>SAPVELVAQPVNAQILPEGEPATPMLGFNGGTPGPVLRARQGEVFDIRFQNQIGEGSAVHWHGLRIDNAMDGVPGMTQDVVEAGGEFEYSFRAPDAGTFWYHSHNRSWEQVAKGLYGPLIVEEPTPPDVDHDLIIMIDDWRITENGVLADGFENMRDQAHQGRLGNFARALVEPVTPVRRGDRV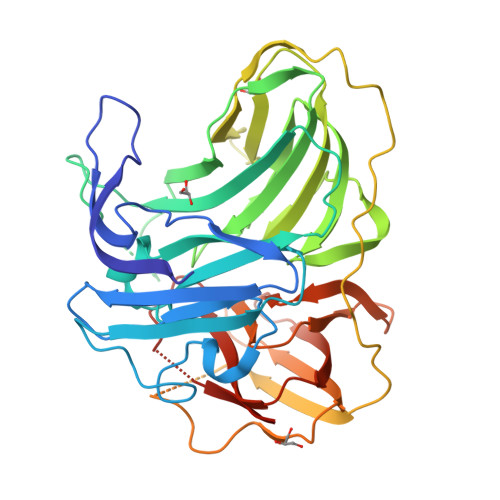RLRLINVATDRIFPVELEGVEGKVVALDGMPIVDPQEFSGLILAPAQRADIIADVITDAPIGFVFPTRDGPYLLGEIPVKGANTTRQPSEIPALPPNEVTSPDMGSAVSLTLTMEGGAMSRRMMQGMMGGDIWAFNGQSGLTDTPLHSFERGQTARIRLVNDTRFPHGIHLHGHHFFEVGADGNLGALRDTTLVDAGETRDIVCVFDNPGNWLLHCHMLGHQAAGMKTWVEVALEHHHHHH[2x]> RVTMNEFEYLKLLGKGTFGKVILVKEKATGRYYAMKILKKEVIVAKDEVAHTLTENRVLQNSRHPFLTALKYSFQTHDRLCFVMEYANGGELFFHLSRERVFSEDRARFYGAEIVSALDYLHSEKNVVYRDLKLENLMLDKDGHIKITDFGLCKEGIKDGATMKTFCGTPEYLAPEVLEDNDYGRAVDWWGLGVVMYEMMCGRLPFY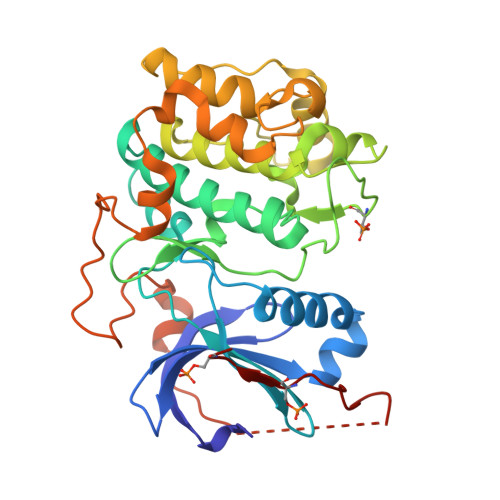NQDHEKLFELILMEEIRFPRTLGPEAKSLLSGLLKKDPKQRLGGGSEDAKEIMQHRFFAGIVWQHVYEKKLSPPFKPQVTSETDTRYFDEEFTAQMITITPPDQDDSMECVDSERRPHFPQFSYSASGTA The yybP–ykoY RNA motif is one of the most widespread riboswitches across bacteria, including many human and plant pathogens. It has evolved to sensitively detect Mn2+ metal ions and broadly regulate a variety of genes, particularly those involved in Mn2+ homeostasis, at the levels of either transcription or translation. The global structure showed that formation of the Mn2+ binding site requires “docking” of two distal helical legs of a four-way junction (4WJ) to form a paperclip-shaped global architecture, facilitated by an A-minor interaction and a second, nonspecific divalent metal ion binding site. The proposed mechanism of transcription antitermination of the yybP–ykoY riboswitch, supported by our structural and dynamic data, involves Mn2+-mediated stabilization of the inherently weak P1.1 switch helix.

In this study, we report the partial and complete Mn2+ dehydration states, captured in the same crystal lattice of the X. oryzae yybP–ykoY riboswitch and resolved to 2.96 Å (Xory-Mn). To facilitate crystallization, the wild-type (WT) Xory sequence was modified distally from the metal ion sensing core not to affect metal ion binding, tightening the 4WJ and stabilizing P1.1 to aid crystallization. The crystal lattice contains two Xory-Mn riboswitch molecules. Conformer 1 is clearly in the canonical Mn2+-sensing state despite minor sequence differences in the metal ion binding core, hence providing a comparable reference point for mechanistic interpretation. Of note, although 80 mM SrCl2 were present in the crystallization buffer, discernible strontium anomalous signals were found in many sites of Xory-conformer 1 but almost none in the MA,Mg site, suggesting that, like Llac-Mn, Xory-conformer 1 prefers smaller divalent ions such as Mg2+ or Mn2+ in MA,Mg. Whereas Xory-conformer 1 serves as a reference point to reveal common themes in Mn2+ sensing among yybP–ykoY riboswitches, Xory-conformer 2 provides a rare, intermediate snapshot of the riboswitch sampling for Mn2+ through a partial dehydration process. Importantly, a partially dehydrated metal ion is already present at the MB,Mn site despite lacking half of the contacts seen in Conformer 1, where only the inner-sphere contacts by the phosphates of A45 and A46 are preserved. Interestingly, the electron density is sufficiently clear to suggest that the invariable adenosine residue (A48) rotates slightly and orients its N1 group closer than N7 towards MB,Mn (a 2.6 Å outer-sphere contact). Importantly, the structural differences observed between the two conformers in the crystal lead us to posit that Conformer 2 with L3 partially unfolded around MB,Mn is likely an intermediate between the fully Mn2+-bound state and the empty MB,Mn state observed in the E. coli Mn2+-free structures.

>[2x]GGCUUGGGGAGUAGCCUGCUUUCGGAAACGAAAGCGCCUGUAUCAACAUACUCGGCGAAAGCCGUGGUGCAGGACCGAAAGGUCUGGCGAGACCAGGCC>[2x]MVRLGPKKPPARKGSMADVPANLMEQIHGLETLFTVSSEKMRSIVKHFISELDKGLSKKGGNIPMIPGWVVEYPTGKETGDFLALDLGGTNLRVVLVKLGGNHDFDTTQNKYRLPDHLRTGTSEQLWSFIAKCLKEFVDEWYPDGVSEPLPLGFTFSYPASQKKINSGVLQRWTKGFDIEGVEGHDVVPMLQEQIEKLNIPINVVALINDTTGTLVASLYTDPQTKMGIIIGTGVNGAYYDVVSGI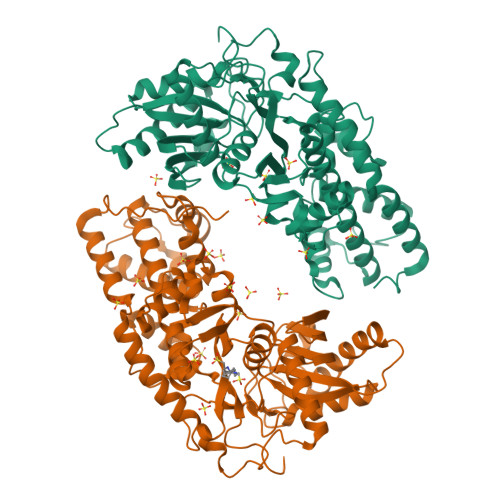EKLEGLLPEDIGPDSPMAINCEYGSFDNEHLVLPRTKYDVIIDEESPRPGQQAFEKMTSGYYLGEIMRLVLLDLYDSGFIFKDQDISKLKEAYVMDTSYPSKIEDDPFENLEDTDDLFKTNLNIETTVVERKLIRKLAELVGTRAARLTVCGVSAICDKRGYKTAHIAADGSVFNRYPGYKEKAAQALKDIYNWDVEKMEDHPIQLVAAEDGSGVGAAIIACLTQKRLAAGKSVGIKGE>[2x]SQLAQWASTRFRSFKRASTLNQDPNTAFYFNKDPIKESLIEMEAELSEEAIKNFSEIMMWM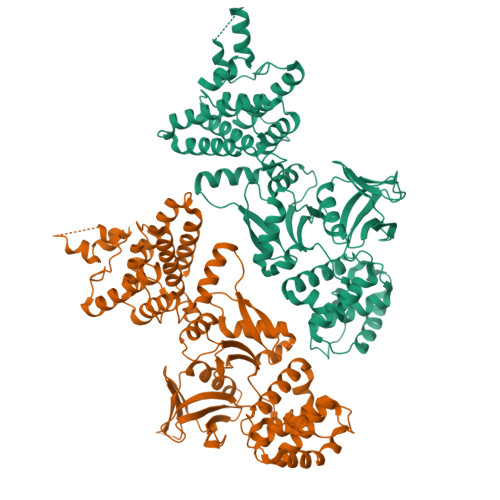GDYPIPKGQTASLVIQSIISRGIENHELRDEIYCQAYRQTNKNPKVESAKKGFELIYFLSITFSPSDSLLQPFMEQLMSRNIAIQSSSPQLASLIAVCIEKLESHPIPSYQQRKMGPSATEIQSFRSNLENGDISTCKIRFIDQSTKLAKINTYTTIREITDTVCRQYGISQQSIKMFGISAVNETAGISKVVSETDMIYDVLARWEQSEEKGEFYFQVRRRFFLDDVNKILDQEHLWTDDDICFELTYCQIRDEWMKGLYTNVNEKDSSIIAAILIQLLYPNQSKLVLTKEVVRQVLPDQILNSQNIKVWISMIESQIFELVSQTPEYLKLMFINLIGSKSPLFGCTLFNIQQKENPPKAWLAINKKGVSIFDPHTKESKNFWTFQSISNVAFTDDTFCIMTGNLMKPIKQTFTTDEHSSIASVYQFYSSQLEH>[9x]PVTLEPMPPGEGAQEGEPPTVEARYKSFSIKMLKDMKEGVKQYGPNSPYMRTLLDSIAHGHRLIPYDWEILAKSSLSPSQFLQFKTWWIDGV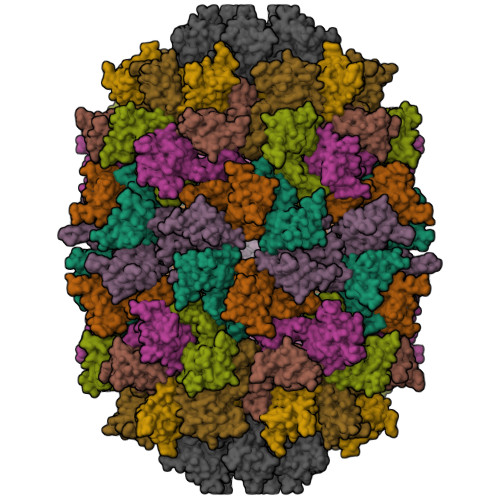QEQVRRNRAANPPVNIDADQLLGIGQNWSTISQQALMQNEAIEQVRAICLRAWEKIQDPGSACPSFNTVRQGSKEPYPDFVARLQDVAQKSIADEKARKVIVELMAYENANPECQSAIKPLKGKVPAGSDVISEYVKACDGIGGAMHKAMLMAQLE>MEAAHSKSTEECLAYFGVSETTGLTPDQVKRHLEKYGHNELPAEEGKSLWELVIEQFEDLLVRILLLAACISFVLAWFEEGEETITAFVEPFVILLILIANAIVGVWQERNAENAIEALKEYEPEMGKVYRADRKSVQRIKARDIVPGDIVEVAVGDKVPADIRILSIKSTTLRVDQSILTGESVSVIKHTEPVPDPRAVNQDKKNMLFSGTNIAAGKALGIVATTGVSTEIGKIRDQMAATEQDKTPLQQKLDEFGEQLSKVISLICVAVWLINIGHFNDPVHGGSWIRGAIYYFKIAVALAVAAIPEGLPAVITTCLALGTRRMAKKNAIVRSLPSVETLGCTSVICSDKTGTLTTNQMSVCKMFIIDKVDGDFCSLNEFSITGSTYAPEGEVLKNDKPIRSGQFDGLVELATICALCNDSSLDFNETKGVYEKVGEATETALTTLVEKMNVFNTEVRNLSKVERANACNSVIRQLMKKEFTLEFSRDRKSMSVYCSPAKSSRAAVGNKMFVKGAPEGVIDRCNYVRVGTTRVPMTGPVKEKILSVIKEWGT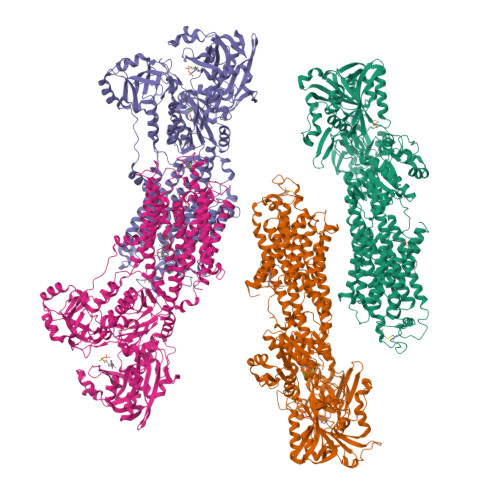GRDTLRCLALATRDTPPKREEMVLDDSSRFMEYETDLTFVGVVGMLDPPRKEVMGSIQLCRDAGIRVIMITGDNKGTAIAICRRIGIFGENEEVADRAYTGREFDDLPLAEQREACRRACCFARVEPSHKSKIVEYLQSYDEITAMTGDGVNDAPALKKAEIGIAMGSGTAVAKTASEMVLADDNFSTIVAAVEEGRAIYNNMKQFIRYLISSNVGEVVCIFLTAALGLPEALIPVQLLWVNLVTDGLPATALGFNPPDLDIMDRPPRSPKEPLISGWLFFRYMAIGGYVGAATVGAAAWWFMYAEDGPGVTYHQLTHFMQCTEDHPHFEGLDCEIFEAPEPMTMALSVLVTIEMCNALNSLSENQSLMRMPPWVNIWLLGSICLSMSLHFLILYVDPLPMIFKLKALDLTQWLMVLKISLPVIGLDEILKFIARNYLEG[4x]>DMEIACLDLEGVLVPEIWIAFAEKTGIDALKATTRDIPDYDVLMKQRLRILDEHGLKLGDIQEVIATLKPLEGAVEFVDWLRERFQVVILSDTFYEFSQPLMRQLGFPTLLCHKLEIDDSDRVVGYQLRQKDPKRQSVIAFKSLYYRVIAAGD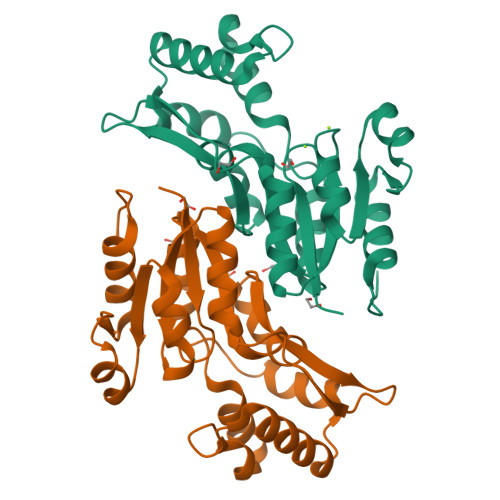SYNDTTMLSEAHAGILFHAPENVIREFPQFPAVHTYEDLKREFLKASSRSLSL[2x]>MAAYTDVPISGMRKTIAARLKESVTENPHFFVSTNLSVSKLLKLRQALNSSADGRYKLSVNDFLIKAMGIASKRVPTVNSSWRDGVIRQFETVDVSVAVATPNGLITPIVKGVEGKGLESISAAVKELAKKARDGKLKPEEYQGGSISISNMGMNPAVQSFTAIINPPQAAILAVGAPQKVAVPVENEDGTTGVSWDEQIIVTASFDHKVVDGAVGAEWIRELKKVIENPLELLL[6x];>HHHHHHSQDPNSSPSSENLYFQSPAPPPVAVVTAPISLSAAIDVQNKLHKTIGVFLPLSTFITRATEIANQKLPLPANYQPTADELFNQVLGLDKVTRKESRGSYTPTFGSFVAPQRAARKADIIDILAAPSTRVAASAQSKSAAPGLTTSGPNVFSLQVPKSEEKRAQAFLQKMKLVLEQEPDKLVRA[3x]

The pyruvate dehydrogenase complex (PDC) is a central metabolic enzyme in all living cells composed majorly of E1, E2, and E3. The 2-oxoacid dehydrogenase complexes are a class of protein complexes with acyl-transferase activity in metabolism and amino acid synthesis. They co-localize 3 catalytic components (E1-3) that act in sequence upon a substrate-carrying lipoyl domain(LD) that is flexibly linked to E2. Like mammals, fungi also utilize E3BP to recruit E321,23–25. The cryo-EM reconstruction of the CBD from N.crassa E3BP inside the PDC core here reveals its oligomeric form and specific interactions.

To determine the interactions of the fungal E3BP:E2 subcomplex, their CBD and CTD respectively were recombinantly co-expressed and examined by cryo-EM. Tetrahedral symmetry was used for the preliminary reconstruction, and 3-fold symmetric sub-complexes were computationally isolated by symmetry expansion and signal subtraction. The final reconstruction to 3.2 Å utilized less than one CBD-trimer per well-aligned PDC core particle, and permits the CBD from N.crassa E3BP to be built de novo. The core fold of the N.crassa CBD consists of four helices and two flanking beta-strands, inherited from an ancestral CTD. The CBD of N.crassa has a trimeric interface with a symmetry axis that coincides with that of a core E2 CTD-trimer. The CBD trimer interface has evolved from the dimeric interface that core CTD trimers form to extend to larger assemblies. It is hydrophobic in nature, formed largely from the C-terminal end of the first CBD helix (residues L285, I289, and V291), as well as it’s C-terminus. The present reconstruction shows unambiguously that M2 is the major binding interface of the E2 core. A conserved Phe (N.crassa F324) appears crucial for binding, as predicted in C.thermophilum. Additionally, K266 from both participating CTD monomers interact with M2 residues N325 and Q326 from the CBD.>MPLCTLRQMLGEARKHKYGVGAFNVNNMEQIQGIMKAVVQLKSPVILQCSRGALKYSDMIYLKKLCEAALEKHPDIPICIHLDHGDTLESVKMAIDLGFSSVMIDASHHPFDENVRITKEVVAYAHARGVSVEAELGTLGGIEEDVQNTVQLTEPQDAKKFVELTGVDALAVAIGTSHGAYKFKSESDIRLAIDRVKTISDLTGIPLVMHGSSSVPKDVKDM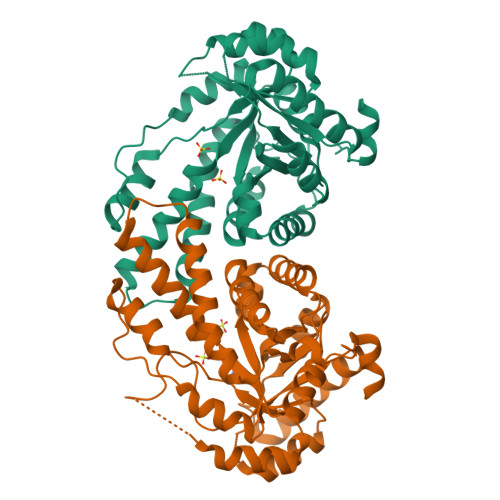INKYGGKMPDAVGVPIESIVHAIGEGVCKINVDSDSRMAMTGAIRKVFVEHPEKFDPRDYLGPGRDAITEMLIPKIKAFGSAGHAGDYKVVSLEEAKAWYK[2x]>[3x]MRHSKRTYCPDWDDKDWDYGKWRSSSSHKRRKRSHSSAQENKRCKYNHSKMCDSHYLESRSINEKD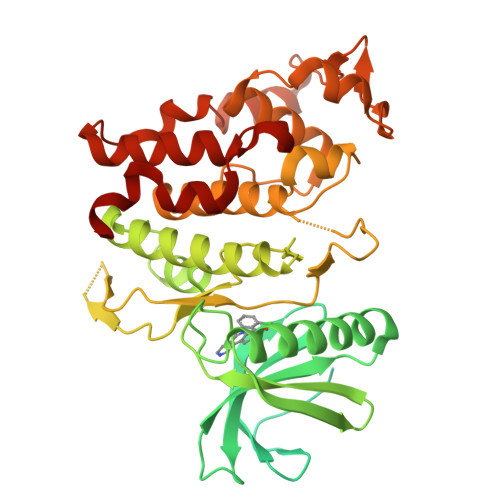YHSRRYIDEYRNDYTQGCEPGHRQRDHESRYQNHSSKSSGRSGRSSYKSKHRIHHSTSHRRSHGKSHRRKRTRSVEDDEEGHLICQSGDVLSARYEIVDTLGEGAFGKVVECIDHKAGGRHVAVKIVKNVDRYCEAARSEIQVLEHLNTTDPNSTFRCVQMLEWFEHHGHICIVFELLGLSTYDFIKENGFLPFRLDHIRKMAYQICKSVNFLHSNKLTHTDLKPENILFVQSDYTEAYNPKIKRDERTLINPDIKVVDFGSATYDDEHHSTLVSTRHYRAPEVILALGWSQPCDVWSIGCILIEYYLGFTVFPTHDSKEHLAMMERILGPLPKHMIQKTRKRKYFHHDRLDWDEHSSAGRYVSRACKPLKEFMLSQDVEHERLFDLIQKMLEYDPAKRITLREALKHPFFDLLKKSI>MPLPKTHELHIFGSFNGVEFDMVGRGIGNPNEGSEELNAKFTKGPLKFSPYILVPHLGYGYYQYLPFPDGMSPFQAAMHDGSGYQVHRTIQYEDGASVTAHYRYTYEGSHIKGEFQVIGTGFPPDGPVMTNKLTAMDWSVTKMLYPNDKTILSTADCSYTTTAGKRYQ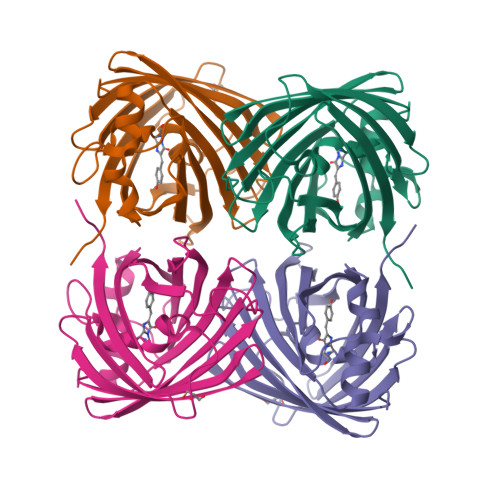SKMRENNTFAKPMAADILQKQPMFVFRKSELQHSKTELTFKEWQKAFTDVMSGGSHHHHHH[8x]> MGMDSSPNEFLNKVIGKKVLIRLSSGVDYKGILSCLDGYMNLALERTEEYVNGK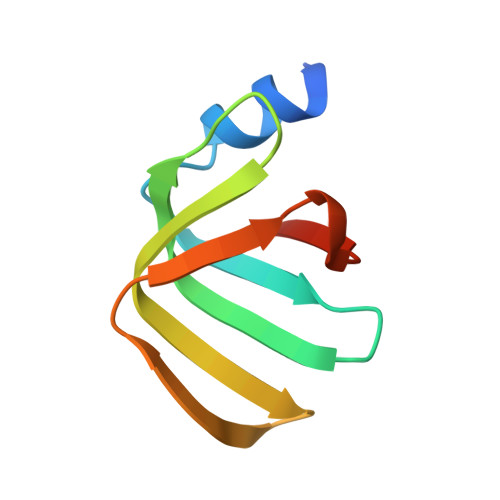KTNVYGDAFIRGNNVLYVSALDD3-[(Z)-AMINO(IMINO)METHYL]-N-[2-(4-BENZOYL-1-PIPERIDINYL)-2-OXO-1-PHENYLETHYL]BENZAMIDE | C28 H28 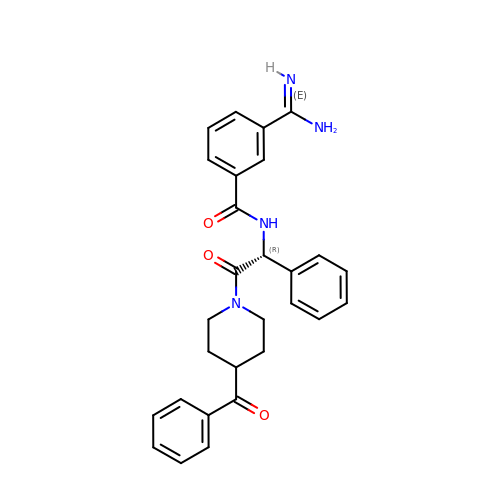N4 O3 | SEXVRUMCMJFNTJ-XMMPIXPASA-N(1R)-9-[(1,3-dimethylazetidin-3-yl)(methyl)amino]-1-methyl-8-phenyl-3,5-dihydro[1,2,4]triazino[3,4-c][1,4]benzoxazin-2(1H)-one 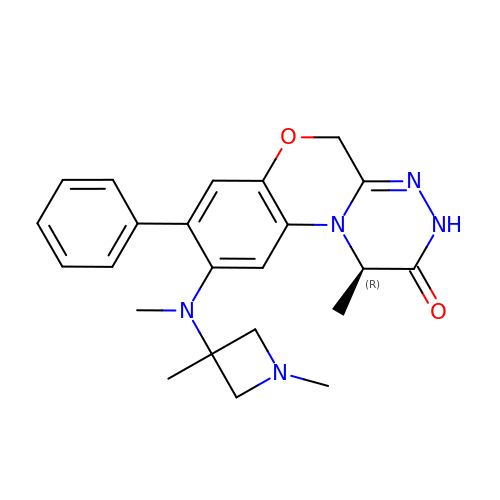| C23 H27 N5 O2 | RGCJJZQGWXZHJQ-OAHLLOKOSA-N> GSMADEATRRVVSEIPVLKTNAGPRDRELWVQRLKEEYQSLI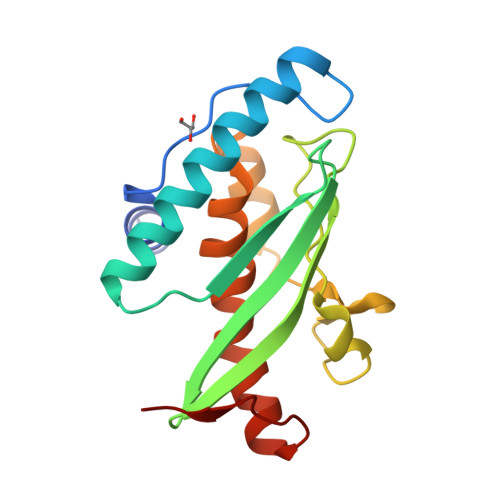RYVENNKNADNDWFRLESNKEGTRWFGKCWYIHDLLKYEFDIEFDIPITYPTTAPEIAVPELDGKIAKMYRGGKICLTDHFKPLWARNVPKFGLAHLMALGLGPWLAVEIPDLIQKGVIHHKEKCNQ>AERGELDLTGAKQNTGVWLVKVPKYLSQQWAKASGRGEVGKLRIAKTQGRTEVSFTLNEDLANIHDIGGKPASVSAPREHPFVLQSVGGQTLTVFTESSSDKLSLEGIVVQRAECRPA[4x];>[4x]AALGPSSQNVTEYVVRVPKNTTKKYNIMAFNAADKVNFATWNQARLERDLSNKKIYQEEEMPESGAGSEFNRKLREEARRKKYGIVLKEFRPEDQPWLLRVNGKSGRKFKGIKKGGVTENTSYYIFTQCPDGAFE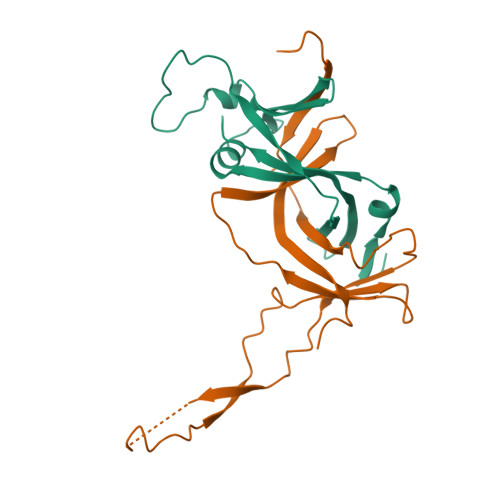AFPVHNWYNFTPLARHRTLTAEEAEEEWERRNKVLN> DLADRFAELERRYDARLGVYVPATGTTAAIEYRADERFAFCSTFAAPLVAAVLHQNPLTHLDKLITYTSDDIRSISPVAQQHVQTGMTIGQLCDAAIRYSDGTAANLLL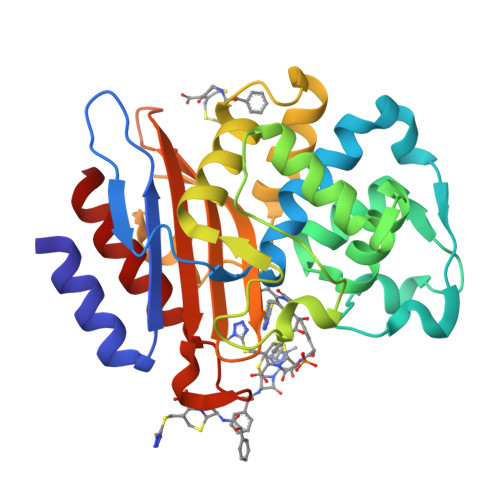ADLGGPGGGTAAFTGYLRSLGDTVSRLDAEEPELNRDPPGDERDTTTPHAIALVLQQLVLGNALPPDKRALLTDWMARNTTGAKRIRAGFPADWKVIDKTGTGDYGRANDIAVVWSPTGVPYVVAVMSDRAGGGYDAEPREALLAEAATCVAGVLA> MTHRFPRSRTALAVALMAGFAMSAQARVFRSADVHGDSFPTNMAVKFMGDELSKLTGGKDSIKVFGNSALGSEKDTVDQVRIGAIDMARVNGASFNEIVPESLIPSFPFLFRDVDHFRKAMYGPAGQKILDAFAAKGMIALTFYESGARSIYAKRPVRTPADMKGLKVRVQPSDLMVDEIRAMGGTPTPMPFAEVYTGLKTGLVDAAENNLPSYEETKHFEVAPDYSETQHAMTPEVLVFSKKIWDTLSPQEQAAIRKAAADSVPYYQKLWTAREASAQQAVTKGGANILPAAQVDRAAFVKAMQPLWTKYEKTPQMKQIVDEIEATKAENLYFQGHHHHHHHHH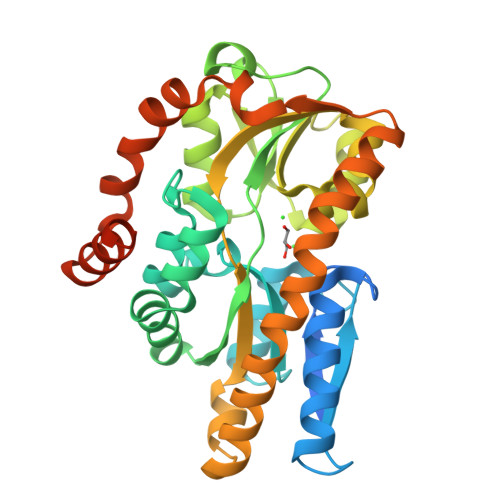H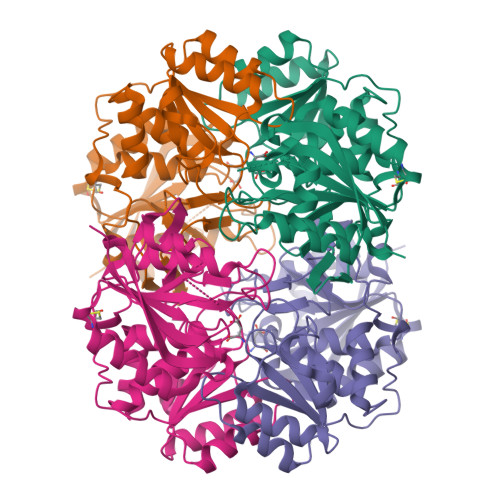>[4x]MDHHHHHHLPNITILATGGVIAGGGDSATKSNYTVGKVGVENLVNAVPQLKDIANVKGEQVVNIGSQDMNDNVWLTLAKKINTDCDKTDGFVITHGTDTMEETAYFLDLTVKCDKPVVMVGAMRPSTSMSADGPFNLYNAVVTAADKASANRGVLVVMNDTVLDGRDVTKTNTTDVATFKSVNYGPLGYIHNGKIDYQRTPARKHTSDTPFDVSKLNELPKVGIVYNYANASDLPAKALVDAGYDGIVSAGVGNGNLYKSVFDTLATAAKTGTAVVRSSRVPTGATTQDAEVDDAKYGFVASGTLNPQKARVLLQLALTQTKDPQQIQQIFNQY>[2x]MRCIGISNRDFVEGVSGGSWVDIVLEHGSCVTTMAKNKPTLDFELIKTEAKQPATLRKYCIEAKLTNTTTESRCPTQGEPTLNEEQDKRFVCKHSMVDRGWGNGCGLFGKGGIVTCAMFTCKKNMEGKIVQPENLEYTVVITPHSGEEHAVGNDTGKHGKEVKITPQSSITEAELTGYGTVTMECSPRTGLDFNEMVLLQMKDKAWLVHRQWFLDLP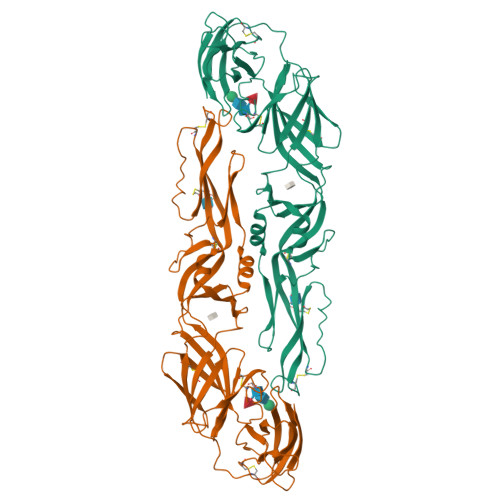LPWLPGADTQGSNWIQKETLVTFKNPHAKKQDVVVLGSQEGAMHTALTGATEIQMSSGNLLFTGHLKCRLRMDKLQLKGMSYSMCTGKFKVVKEIAETQHGTIVIRVQYEGDGSPCKIPFEIMDLEKRHVLGRLITVNPIVTEKDSPVNIEAEPPFGDSYIIIGVEPGQLKLNWFKK O5'-(L-GLUTAMYL-SULFAMOYL)-ADENOSINE 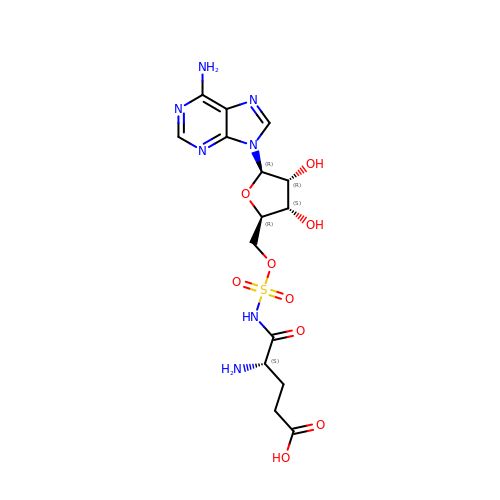| C15 H21 N7 O9 S | YBRKRYFZKHICLS-WERHYGNASA-N>MEGLAGYVYKAASEGKVLTLAALLLNRSESDIRYLLGYVSQQGGQRSTPLIIAARNGHAKVVRLLLEHYRVQTQQTGTVRFDGYVIDGATALWCAAGAGHFEVVKLLVSHGANVNHTTVTNSTPLRAACFDGRLDIVKYLVENNANISIANKYDNTCLMIAAYKGHTDVVRYLLEQRADPNAKAHCGATALHFAAEAGHIDIVKELIKWRAAIVVNGHGMTPLKVAAESCKADVVELLLSHADCDRRSRIEALELLGASFANDRENYDIIKTYHYLYLAMLERFQDGDNILEKEVLPPIHAYGNRTECRNPQELESIRQDRDALHMEGLIVRERILGADNIDVSHPIIYRGAVYADNMEFEQCIKLWLHALHLRQKGNRNTHKDLLRFAQVFSQMIHLNETVKAPDIECVLRCSVLEIEQSMNRVKNISDADVHNAMDNYECNLYTFLYLVCISTKTQCSEEDQCKINKQIYNLIHLDPRTREGFTLLHLAVNSNTPVDDFHTNDVCSFPNALVTKLLLDCGAEVNAVDNEGNSALHIIVQYNRPISDFLTLHSIIISLVEAGAHTDMTNKQNKTPLDKSTTGVSEILLKTQMKMSLKCLA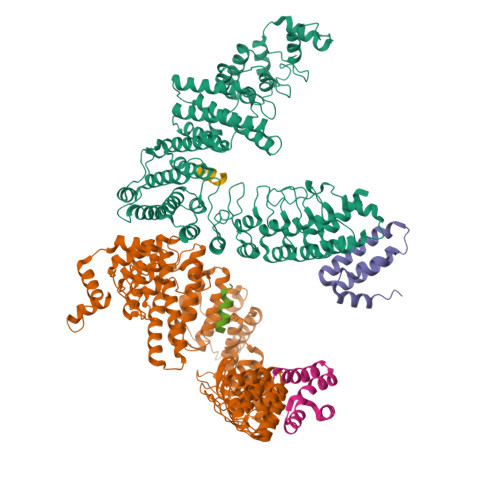ARAVRANDINYQDQIPRTLEEFVGFH[2x];>DRKRRSDPNFKNRLRERRKKQKLAKERAGLSKLPDLKDAEAVQKFFLEEIQLGEELLAQGEYEKGVDHLTNAIAVCGQPQQLLQVLQQTLPPPVFQMLLTKLPTISQRIVSAQSLAEDDVE[2x]>[2x]ANFIEKITYLGTPAIKAGNEHLEMIVVPEWGSNVISLVDKTTNVQLLREPETAESFHDTPTLYGIPILFPPNRISDGTFSFRGRTYHFDINEKDKHNHLHGFLYHEKWNVVTTKQTDEGVIVETEIDLSELPHVQKQFPHHAVVRMTYTIKENTLFKHATVMNKGKEAFPWGIGYHTTFIFPAESSLFSLTADQQWELDERLLPTGKLMDVPYKEALHEGMDLRHKQLDDV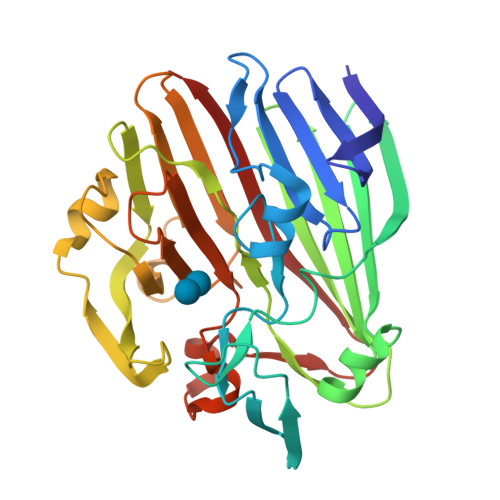FLSSYQKRGGENQAVIYHQHAHISIIYKADEQFKHWVVYNADGKQGYLCPEPYTWVTNAVNLDLPSSLTGLQVLEPGEETTAKSSITIELNHQ> MFLYTETDQNLQA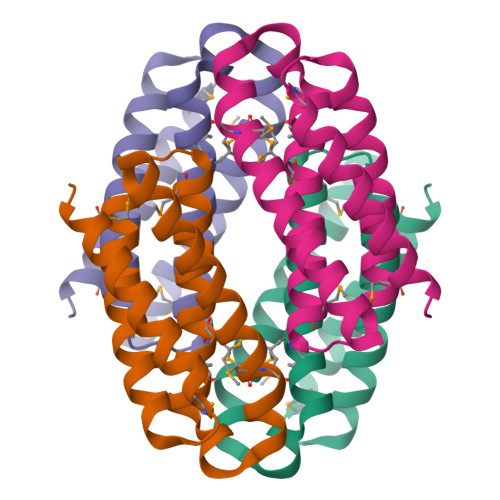CIDACNHCYRTCLRMAMNHCLEAGGKHVEADHLRLMMNCAEICQTSLNFMLSGSRFSPKVCGVCAEICDACAKSCEQLDGMEECVQTCRQCAEHCRKMAALEHHHHHH In the human fungal pathogen Candida albicans, ARO1 encodes an essential multi-enzyme that catalyses consecutive steps in the shikimate pathway for biosynthesis of chorismate, a precursor to folate and the aromatic amino acids. In Fungi and Apicomplexa, the second to the sixth steps of the shikimate pathway are supported by five enzymatic domains combined in a single protein known as Aro1 or AroM. Aro1 forms a flexible dimer allowing relative autonomy of enzymatic function of the individual domains. Our activity and in cellulo data suggest that only four of Aro1’s enzymatic domains are functional and essential for viability of C. albicans, whereas the 3-dehydroquinate dehydratase (DHQase) domain is inactive because of active site substitutions.

We performed local refinement on the dimer of the Aro1SK-DHQase-DHSD region, as well as the dimer of Aro1DHQS and Aro1EPSPS domains that resulted in molecular maps of resolutions of 3.16 Å for Aro1SK-DHQase-DHSD and 3.43 Å for Aro1DHQS-EPSPS. In this map, we performed only a rigid body fit of two high-resolution models for Aro1DHQS-EPSPS and Aro1SK-DHQase-DHSD domains. These two models (Aro1DHQS-EPSPS and Aro1SK-DHQase-DHSD) were obtained by docking and refining against cryo-EM maps X-ray crystallographic models described earlier. Within these particles, there was further structural heterogeneity, due to the Aro1SK-DHQase-DHSD fragment tilting in various conformations relative to the Aro1DHQS domain. There are additional contacts between the Aro1DHQase domains in the Aro1 dimer that may also contribute to dimerization. The Aro1DHQS domain, Aro1EPSPS subdomain II, and Aro1SK-DHQase-DHSD backbones show nearly identical conformation within the core structure of each region with minor differences seen in some loop regions.

>[2x]MSIEKVPILGKETIHVGYGIADHIVREVIANLASSTYVIVTDTNMARTPQYSKLTDDFKTNLSEKRPESRLLTYCVSPGENNKNRATKAAVEDFLLQQGCTRDTVILAVGGGVIGDMIGFVAATFMRGVRVVQVPTTLLAMVDSSVGGKTAIDTPLGKNFIGAFHQPEYVFCDVSFLETLPARQFINGMAEVVKTAAIWNEEEFTRLENFSKKFLSVVTSKKPDLQSIKAELVKTVLESVRVKAGVVSSDEKEAGLRNLLNFGHTIGHAIEAVLTPEALHGECVSIGMIKEAELSRYLGILPPVAVARLSKCLVAYGLPVSIDDKEFLKKVGPKRHYVEIDILLKKMAIDKKNDGSKIRCVLLEKIGKCYQLKAHQVSKQDLSFVLTDEVLVHPFTNPPKENIIVPPGSKSISNRALILAALGNGTVRVKNLLHSDDTKHMLDAVASLKGAEISTEDNGETIVVKGNGGNLVTSGEELYLGNAGTASRFLTTVASLVGKSQASDDVILTGNARMQERPIGPLVDALGSNGSEIEYLNKQGSLPLKISAGNGLKGGRIELAATISSQYVSSILMCAPYAKEPVTLALVGGKPISQLYIDMTCAMMKSFGIEVTKSTTEEYTYHIPKGTYKNPSEYVIESDASSATYPLAFAAMTGTSCTIPNIGSSSLQGDAKFAVDVLKPMGCKVEQTTTSTTVTGPPRGHLKPLPHVDMEPMTDAFLTASVVAAVAKGGSSTSITGIANQRVKECNRIEAMVTELAKFGVPANELPDGIEIHGIDIEDLKTPEISKRGVSSYDDHRVAMSFSLLAGLCKEPVLILERSTTGKTWPGWWDILHSKFKIELDGYEPPFNTDKHVDKSSDKSIIVIGMRGTGKSTLSEWLASFLGFKMLDMDKYLEEKLGTGIKSLIKAKGWEYFRQEEAIVAKECFTKFSKGYVLSTGGGIVEGEDARQQLKSYADNGGIVLHLHRDLDETVTFLAADTTRPAYSSEVQEVWLRREKWYHECSNYHFYSSHCSTEDEFNHLRRSFVNYIKLITGAERPVVPAGRSAAVVLTSPDLNEVVGDLESITIGADAVELRVDLFKDTSAEFVAAQIAVIRKHADLPIIYTVRTVSQGGKFPDENVDELKSLLLLGIRLGVAYVDLQLTAPNELIEEISSKKGFTRVIGTYQDINGELKWNNVEWKNKYNQGVSMNADIVRLVGKANSIQDNLDLENFKKQNTLKPLIAFNLGSQGKLSQVLNGTFTPISHKLLPNDEEFLTIGELNQTYFDIGGFTAKKFWVIGSPIEHSRSPNLHNAGYKALNLPYQFGRFEATDVDVVYDNLINKPDFGGLAITMPLKLDIMKFATKLSDAAETIGAVNTLIPIEGGYFGDNTDWVGISNSFIRAGVPPKSSSNGLVVGAGGTSRAAIYALHQMGCAKIYLVNRTAAKLEELVKSFPKDYNLEIVETEQQADKASKVSLAVSCIPADKPLDGEVLKKIERILSNGSEQSAGFKPTLLEASYKPRVTPIMKLTEEQYKWKVIPGVEMLVNQGDRQFKLHTGFTAPYEIIHRAVVEE> KEKHYYIGIIETTWDYASDHGEKKLISVDTEHSNIYLQNGPDRIGRLYKKALYLQYTDETFRTTIEKPVWLGFLGPIIKAETGDKVYVHLKNLASRPYTFHSHGITYYKEHEGAIYPDNTTDFQRADDKVYPGEQYTYMLLATEEQSPGEGDGNCVTRIYHSHIDAPKDIASGLIGPLIICKKDSLDKEKEKHIDREFVVMFSVVDENFSWYLEDNIKTYCSEPEKVDKDNEDFQESNRMYSVNGYTFGSLPGLSMCAEDRVKWYLFGMGNEVDVHAAFFHGQALTNKNYRIDTINLFPATLFDAYMVAQNPGEWMLSCQNLNHLKAGLQAFFQVQECNKSSSKDNIRGKHVRHYYIAAEEIIWNYAPSGIDIFTKENLTAPGSDSAVFFEQGTTRIGGSYKKLVYREYTDASFTNRKERGPEE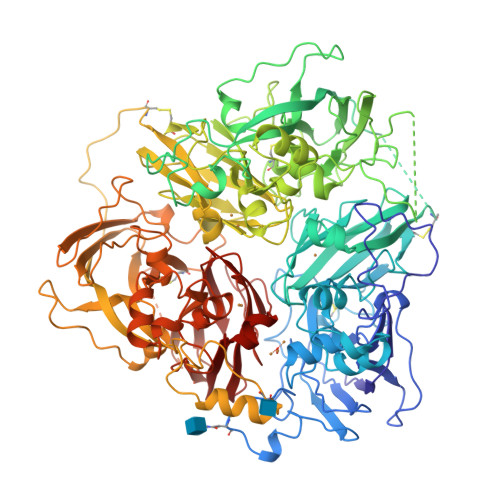EHLGILGPVIWAEVGDTIRVTFHNKGAYPLSIEPIGVRFNKNNEGTYYSPNYNPQSRSVPPSASHVAPTETFTYEWTVPKEVGPTNADPVCLAKMYYSAVDPTKDIFTGLIGPMKICKKGSLHANGRQKDVDKEFYLFPTVFDENESLLLEDNIRMFTTAPDQVDKEDEDFQESNKMHSMNGFMYGNQPGLTMCKGDSVVWYLFSAGNEADVHGIYFSGNTYLWRGERRDTANLFPQTSLTLHMWPDTEGTFNVECLTTDHYTGGMKQKYTVNQCRRQSEDSTFYLGERTYYIAAVEVEWDYSPQREWEKELHHLQEQNVSNAFLDKGEFYIGSKYKKVVYRQYTDSTFRVPVERKAEEEHLGILGPQLHADVGDKVKIIFKNMATRPYSIHAHGVQTESSTVTPTLPGETLTYVWKIPERSGAGTEDSACIPWAYYSTVDQVKDLYSGLIGPLIVCRRPYLKVFNPRRKLEFALLFLVFDENESWYLDDNIKTYSDHPEKVNKDDEEFIESNKMHAINGRMFGNLQGLTMHVGDEVNWYLMGMGNEIDLHTVHFHGHSFQYKHRGVYSSDVFDIFPGTYQTLEMFPRTPGIWLLHCHVTDHIHAGMETTYTVLQNEDTKSG>[2x]MITSPTNLNSLPIPPGDFGLPWLGETLNFLNDGDFGKKRQQQFGPIFKTRLFGKNVIFISGALANRFLFTKEQETF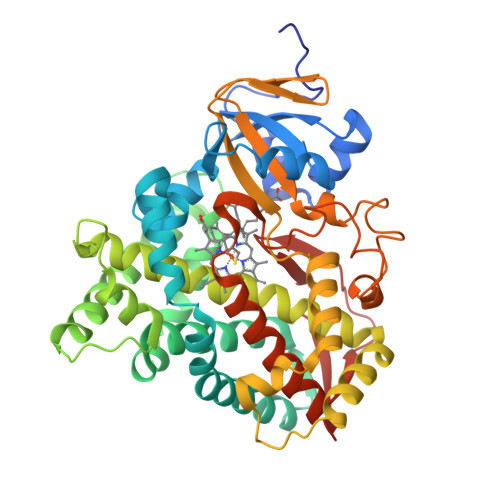QATWPLSTRILLGPNALATQMGEIHRSRRKILYQAFLPRTLDSYLPKMDGIVQGYLEQWGKANEVIWYPQLRRMTFDVAATLFMGEKVSQNPQLFPWFETYIQGLFSLPIPLPNTLFGKSQRARALLLAELEKIIKARQQQPPSEEDALGILLAARDDNNQPLSLPELKDQILLLLFAGHETLTSALSSFCLLLGQHSDIRERVRQEQNKLQLSQELTAETLKKMPYLDQVLQEVLRLIPPVGGGFRELIQDCQFQGFHFPKGWLVSYQISQTHADPDLYPDPEKFDPERFTPDGSATHNPPFAHVPFGGGLRECLGKEFARLEMKLFATRLIQQFDWTLLPGQNLELVVTPSPRPKDNLRVKLHSLM>MMNVMLPAPDLYSLSFIHITRISYMKTLSQNTTSSACAPETGLQQLVATIVPDEQRISFWPQHFGLIPQWVTLEPRVFGWMDRLCENYCGGIWNLYTLNNGGAFMAPEPDDDDDETWVL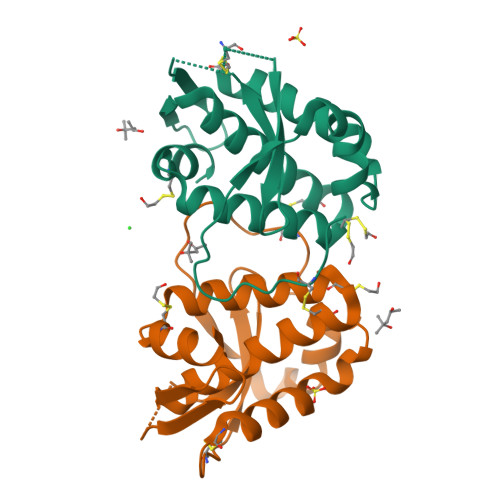FNAMNGNRAEMSPEAAGIAACLMTYSHHACRTECYAMTVHYYRLRDYALQHPECSAIMRIID[2x]>MGSETETVTVEGIPFPAEITFTAGGNPAVSLVGNGITDIEIHFLQIKYNAIGIYLHSNDVLLDHLHGWKGKSADELLGDDSFFQALVAAPVEKLFRVVVIKEIKGSQYGVQLESSVRDRLVAADKYDDDEEEALEKITDFFQAKYFKPGSVITFHFPATSAAGAVEISFATEGKDAAKMKVENENVARMIQKWYLGGDSAVSPTTVRSMADRF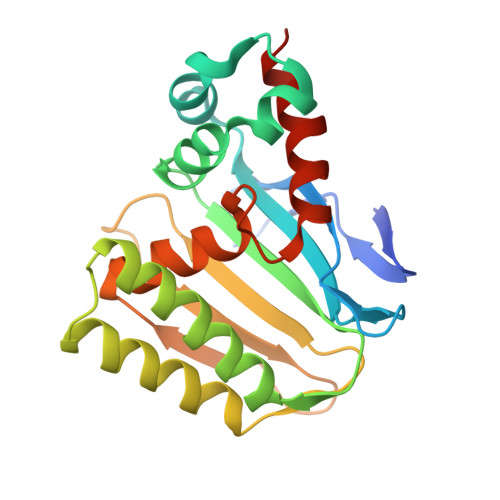AALLSAASEF[2x]>[4x]TYERTFVKKDAETKEVL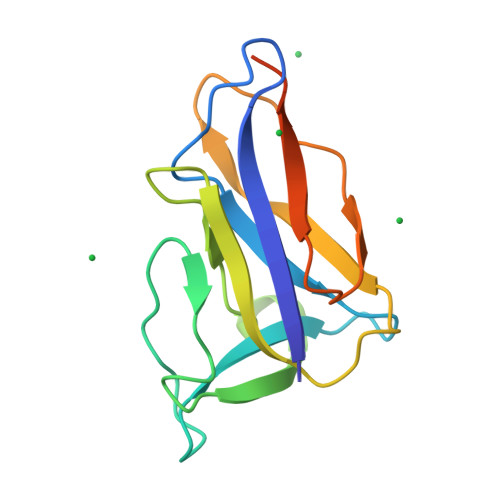EGAGFKISNSDGKFLKLTDKDGQSVSIGEGFIDVLANNYRLTWVAESDATVFTSDKSGKFGLNGFADNTTTYTAVETNVPDGYDAAANTDFKADNSSSDILDAPSGILPLEHHHHHH>[2x]SNAMETGDQRFGDLVFRQLAPNVWQHTSYLDMPGFGAVASNGLIVRDGGRVLVVDTAWTDDQTAQILNWIKQEINLPVALAVVTHAHQDKMGGMDALHAAGIATYANALSNQLAPQEG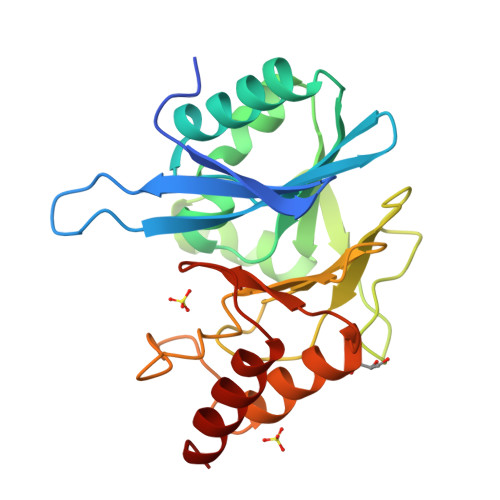MVAAQHSLTFAANGWVEPATAPNFGPLKVFYPGPGHTSDNITVGIDGTDIAFGGCLIKDSKAKSLGNLGDADTEHYAASARAFGAAFPKASMIVMSHSAPDSRAAITHTARMADKLR> MAAQIPESDQIKQFKEFLGTYNKLTETCFLDCVKDFTTREVKPEETTCSEHCLQKYLKMTQ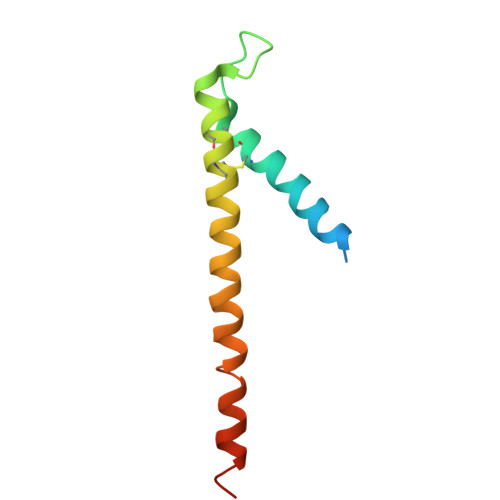RISMRFQEYHIQQNEALAAKAGLLGQPR> PVNLNNLEAKRIVACDDPDFLTSYFAHSRLHHLSAWKANLKDKFLNENIHKYTKITDKDTYIIFHIDFDCFFATVAYLCRSSSFSACDFKRDPIVVCHGTKNSDIASCNYVARSYGIKNGMWVSQAEKMLPNGIKLISLPYTFEQFQLKSEAFYSTLKRLNIFNLILPISIDEAVCVRIIPDNIHNTNTLNARLCEEIRQEIFQGTNGCTVSIGCSDSLVLARLALKMAKPNGYNITFKSNLSEEFWSSFKLDDLPGVGHSTLSR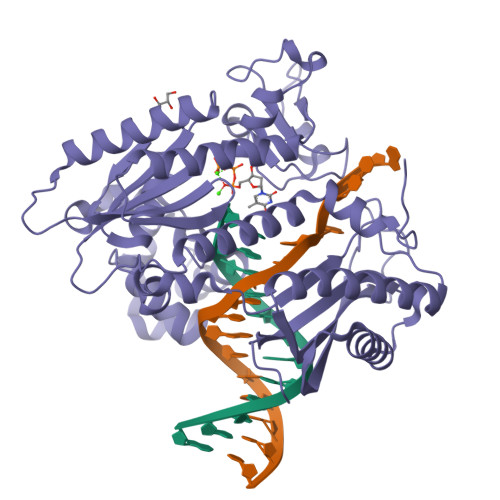LESTFDSPHSLNDLRKRYTLDALKASVGSKLGMKIHLALQGQDDEESLKILYDPKEVLQRKSLSIDINWGIRFKNITQVDLFIERGCQYLLEKLNEINKTTSQITLKLMRRCKDAPIEPPKYMGMGRCDSFSRSSRLGIPTNEFGIIATEMKSLYRTLGCPPMELRGLALQFNKLVDVGPDNNQLK>[2x]MMSETA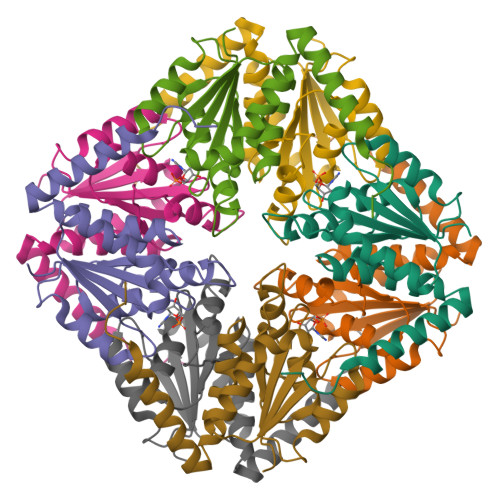PLPSASSALEDKAASAPVVGIIMGSQSDWETMRHADALLTELEIPHETLIVSAHRTPDRLADYARTAAERGLNVIIAGAGGAAHLPGMCAAWTRLPVLGVPVESRALKGMDSLLSIVQMPGGVPVGTLAIGASGAKNAALLAASILALYNPALAARLETWRALQTASVPNSPITEDK> SVSFYEIANGNEVHT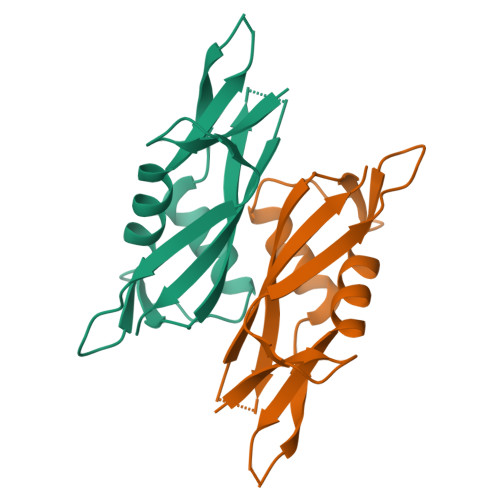GSLNMTANPTSHELNVSAVLAAAKAKYAAHQLENGASNGASVAVTTDVKDLTDQLTKAGIKVDPLGNFQAQASFSFNLAAKSAQNAATATLPITVSVAN> IY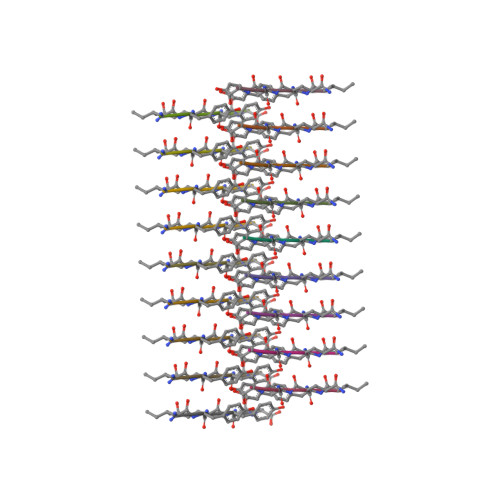QYGG>[2x]MSLYKRKSKLIGLL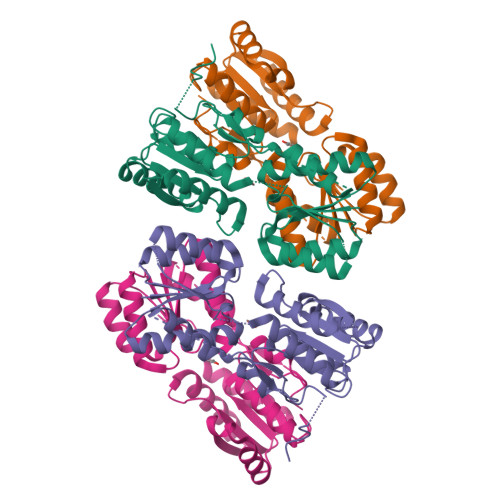LPDMSNPFFTLIARGVEDVALAHGYQVLIGNSDNDIKKAQGYLATFVSHNCTGMISTAFNENIIENTLTDHHIPFVFIDRINNEHNGISTNHFKGGQLQAEVVRKGKGKNVLIVHENLLIDAFHQRVQGIKYILDQQRIDYKMLEATLLDNDKKFIDLIKELSIDSIICSNDLLAINVLGIVQRYHFKVPAEIQIIGYDNIPFSEMTYPQITTIDQSAYHLGEIAVSQLLGLNTDNLTNNHKQLALTVKHRGSTREGHHHHHH TYROSINE | C9 H11 N O3 | 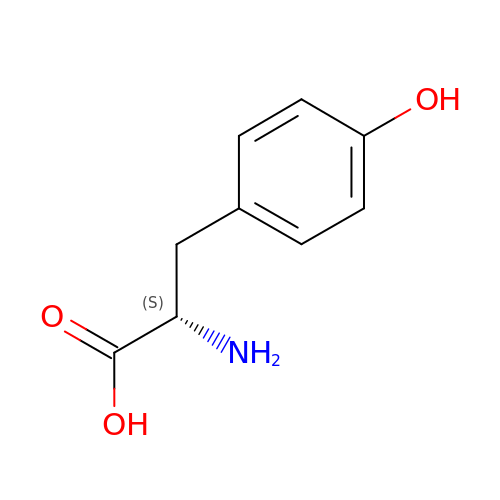OUYCCCASQSFEME-QMMMGPOBSA-N> MAEQVALSRTQVCGILREELFQGDAFHQSDTHIFIIMGASGDLAKKKIYPTIWWLFRDGLLPENTFIVGYARSRLTVADIRKQSEPFFKATPEEKLKLEDFFARNSYVAGQYDDAASYQRLNSHMNALHLGSQANRLFYLALPPTVYEAVTKNIHESCMSQIGWNRIIVEKPF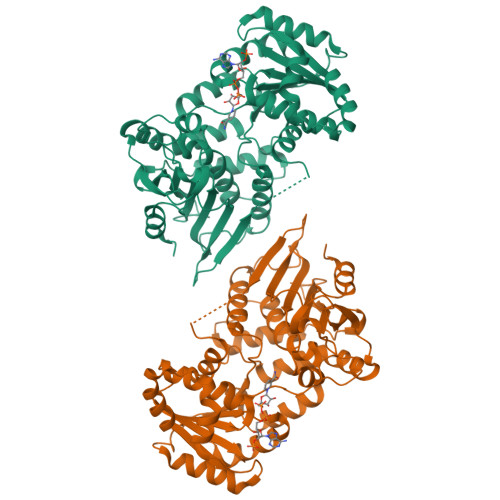GRDLQSSDRLSNHISSLFREDQIYRIDHYLGKEMVQNLMVLRFANRIFGPIWNRDNIACVILTFKEPFGTEGRGGYFDEFGIIRDVMQNHLLQMLCLVAMEKPASTNSDDVRDEKVKVLKCISEVQANNVVLGQYVGNPDGEGEATKGYLDDPTVPRGSTTATFAAVVLYVENERWDGVPFILRCGKALNERKAEVRLQFHDVAGDILHQQCKRNELVIRVQPNEAVYTKMMTKKPGMFFNPEESELDLTYGNRYKNVKLPDAYERLILDVFCGSQMHFVRSDELREAWRIFTPLLHQIELEKPKPIPYIYGSRGPTEADELMKRVGFQYEGTYKWVNPHKL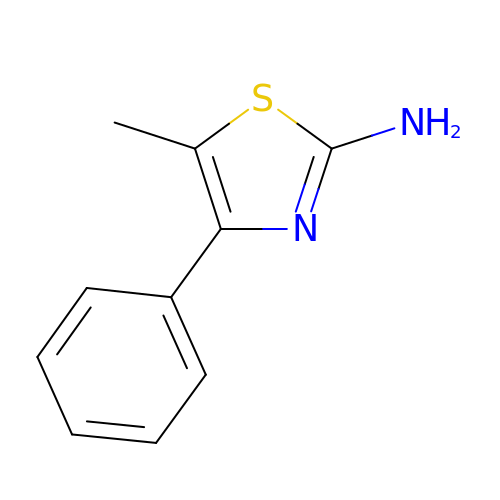5-methyl-4-phenyl-1,3-thiazol-2-amine | C10 H10 N2 S | HTXQOROHFFYFMC-UHFFFAOYSA-N> MVSAKDFSGAELYTLEEVQYGKFEARMKMAAASGTVSSMFLYQNGSEIADGRPWVEVDIEVLGKNPGSFQSNIITGKAGAQKTSEKHHAVSPAADQAFHTYGLEWTPNYVRWTVDGQEVRKTEGGQ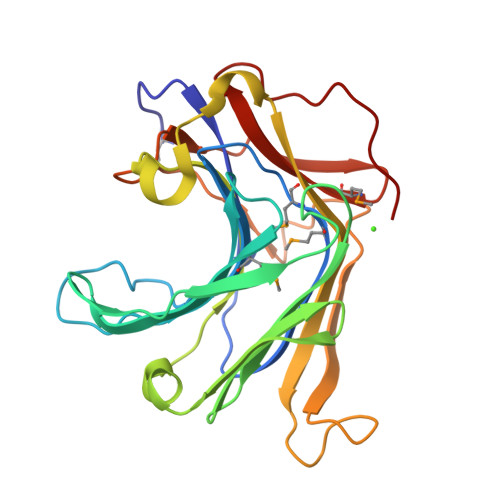VSNLTGTQGLRFNLWSSESAAWVGQFDESKLPLFQFINWVKVYKYTPGQGEGGSDFTLDWTDNFDTFDGSRWGKGDWTFDGNRVDLTDKNIYSRDGMLILALTRKGQESFNGQVPRD>MEILHDEDVDDSILRDKTIAVMGYGAQGDAQANCLKDSGINVVIGETEILGGNKNPSWEKAKEDGFEVLPIDKAAEKGDVVHILLPDEVQPAIYENQIKPQLKAGKALCFSHGFNICFKRIVPPEDVDVIMVAPKAPGTEERKAYLEGFGVPGLVAVKQNPSGEAREVALAMTKAMHWTKAGILECTFEQETYEDLFGEQCVLCGGLVELMRNGFEVLVEAGYPPEMAYFECVHEMKLIVDLVWQGGIKRMAEVISNTAEYGMWAVGHQIIGPEVKEKMKEALKRVENGEFANEWVD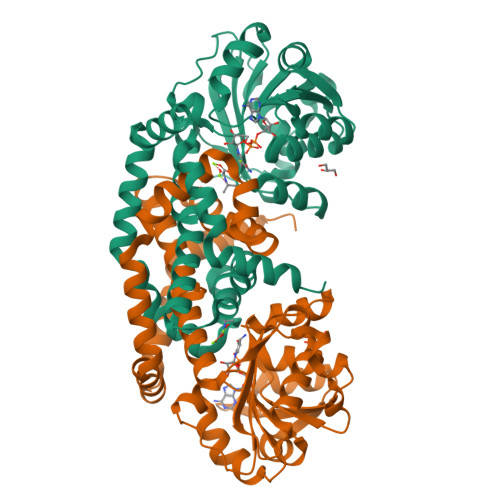EYKRGIPFLKASREKMGEHQVETVGAEIRKLFAQKHHHHHH[2x]> AMPFEIEVLLPGEISPAETSALQKCEGKIITFSTLRHRASLVDIALSSYYINGAPPDTLSLLEAYRMRFAAVITRVIPGKLLAHAIGVGTPTPGLFIQNTSPVDLCNGDYICLLPPVFGSADEIRLDSVGLEIVFPLTIPQTL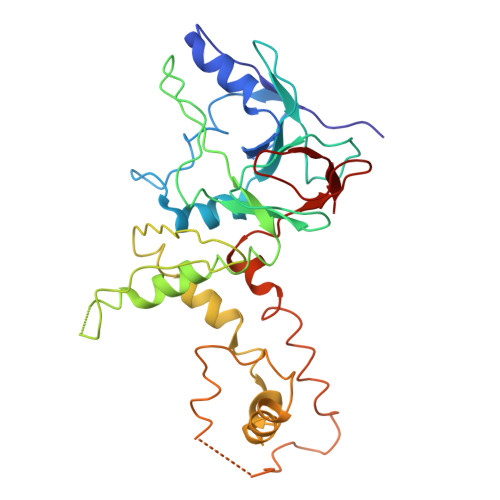MREIIAKVVARAVERTAAGRTPGELPGADVICYNGRRYELETNLQHRDGSDAAIRTLVLNLMFSINEGTTLILTLITRLLVQGAHDGYVNLLIQTANCVRETGQPMPRIQDGHRRFPIYEAISSWISTSSRLGDTLGTRAILRVCVFDGPSTVHPGDRTAVIQV>[2x]MAETR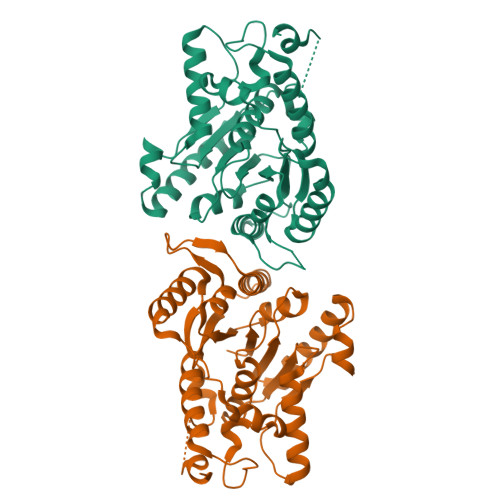VIVVGNEKGGAGKSTIAVHLVTALLYGGAKVAVIDLDLRQRTSARFFENRRAWLDNKKIELPEPLALNLSDNDVALAERPEEEQVAGFEAAFARAMAECDFILIDTPGGDSAITRMAHGRADLVVTPMNDSFVDFDMLGTVDPVTLELTKPSLYSLTVWEGRKQRALSGQRQAMDWVVLRNRLATTEARNRKRLEDRLNALAKRVGFRIGPGLRDRVIYRELFPFGLTIADLSPQVRPVPVSLQHLAARQELRALMHSLGLSAYSGETMLAAQAVDKLAAALEHHHHHH>METFTVKMGADSGLLQFEPANVTVHPGDTVKWVNNKLPPHNILFDDKQVPGASKELADKLSHSQLMFSPGESYEITFSSDFPAGTYTYYCAPHRGAGMVGKIT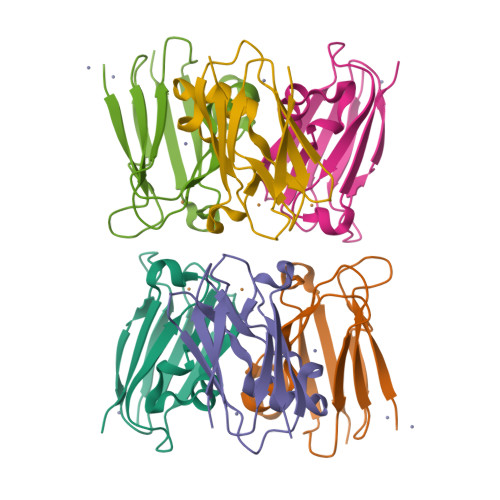VEG[3x]>[6x]MSNNEFHQRRLSATPRGVGVMCNFFAQSAENATLKDVEGNEYIDFAAGIAVLNTGHRHPDLVAAVEQQLQQFTHTAYQIVPYESYVTLAEKINALAPVSGQAKTAFFTTGAEAVENAVKIARAHTGRPGVIAFSGGFHGRTYMTMALTGKVAPYKIGFGPFPGSVYHVPYPSDLHGISTQDSLDAIERLFKSDIEAK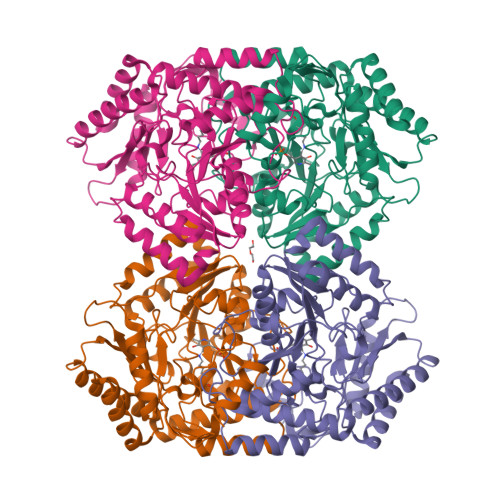QVAAIIFEPVQGEGGFNVAPKELVAAIRRLCDEHGIVMIADEVQSGFARTGKLFAMDHYADKPDLMTMAKSLAGGMPLSGVVGNANIMDAPAPGGLGGTYAGNPLAVAAAHAVLNIIDKESLCERANQLGQRLKNTLIDAKESVPAIAAVRGLGSMIAVEFNDPQTGEPSAAIAQKIQQRALAQGLLLLTCGAYGNVIRFLYPLTIPDAQFDAAMKILQDALSD>[4x]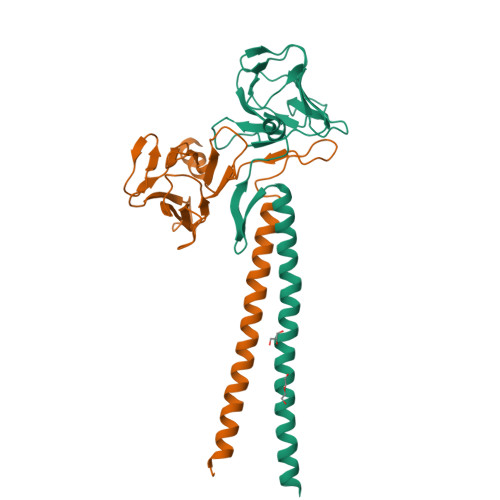GPGSEFSEEAIERLKETEKIIAELNETWEEKLRRTEAIRMEREALLAEMGVAMREDGGTLGVFSPKKTPHLVNLNEDPLMSECLLYYIKDGITRVGREDGERRQDIVLSGHFIKEEHCVFRSDSRGGSEAVVTLEPCEGADTYVNGKKVTEPSILRSGNRIIMGKSHVFRFNHPEQARQERERT>[6x]MAKNNAVAGFNALNGVELNLFTTDELKAIHYATMEVLMDPGIQVSDPEARQIFKENGCEVNEKTNVVKIPEYLVRKALQLAPSRFVLWGRDKKFNTVQECGGKVHWTCFGTGVKVCKYQDGKYVTVDSVEKDIADIAKLCDWAENIDYFSLPVSARDIAGQGAQDVHETLTPLANTAKHFHHIDPVGENV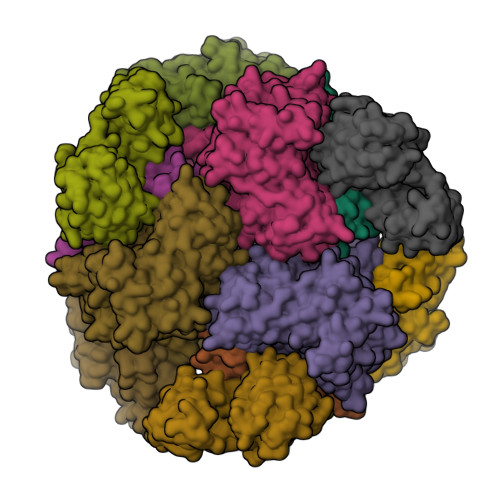EYYRDIVKAYYGGDEEEARKKPIFSMLLCPTSPLELSVNACQVIIKGARFGIPVNVLSMAMSGGSSPVYLAGTLVTHNAEVLSGIVLAQLTVPGAKVWYGSSTTTFDLKKGTAPVGSPELGLISAAVAKLAQFYGLPSYVAGSOSDAKVPDDQAGHEKTMTTLLPALAGANTIYGAGMLELGMTFSMEQLVIDNDIFSMVKKAMQGIPVSEETLAVESIQKVGIGNNFLALKQTRQLVDYPSNPMLLDRHMFGDWAAAGSKDLATVAHEKVEDVLKNHQVTPIDADIFKDMQAIVDKADKAFRGMGGHHHHHH;>MANKEEIIAKAKEAITDFDDELAEEVANEALAAGIDPVELIEKGFTAGMEEVGEKFGQGELFLPHVLAAAEAMNSGIKVITPEMEKRKSQTKSLGTVAIGTIEGDIHSIGKDIVASMLNIAGFKVVDLGRDVPINTFVEKVKELKPQVVASSALMTTTMVNQIQIEEQLKEAGVRDQVKTMVGGAPVTQDWADKIGADIYGESANDAVAKVKAALNVGGHHHHH[6x]>[12x]MRITTKVGDKGSTRLFGGEEVWKDSPIIEANGTLDELTSFIGEAKHYVDEEMKGILEEIQNDIYKIMGEIGSKGKIEGISEERIAWLLKLILRYMEMVNLKSFVLPGGTLESAKLDVCRTIARRALRKVLTVTREFGIGAEAAAYLLALSDLLFLLARVIEIE;>[12x]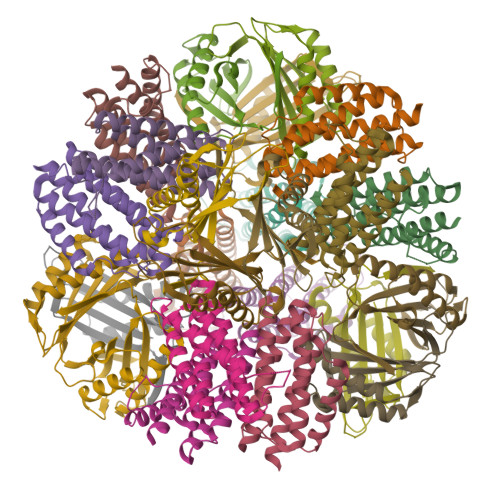MPHLVIEATANLRLETSPGELLEQANKALFASGQFGEADIKSRFVTLEAYRQGTAAVERAYLHACLSILDGRDIATRTLLGASLCAVLAEAVAGGGEEGVQVSVEVREMERLSYAKRVVARQRLEHHHHHH MukBEF folds the chromosome of Escherichia coli and related bacteria. The SMC protein MukB dimerizes at its ‘‘hinge’’ domain, which connects via the long coiled-coil ‘‘arm’’ to the ABC-type ATPase ‘‘head’’ domain. The heads are bridged by the kleisin MukF, whereby the C-terminal winged-helix domain (cWHD) of MukF binds the ‘‘cap’’ surface of one MukB, and the N-terminal middle domain (MD) binds the coiled-coil ‘‘neck’’ of the other MukB. MukF also recruits the dimeric KITE protein MukE.

MukBEF is an obligate dimer, formed by two MukB2E2F monomers held together by their MDs and MukF N-terminal winged-helix domains (nWHDs). Focused sub-classification of the particle images revealed a DNA-bound structure. The DNA was captured directly at the open gate, while the proteins adopted a conformation virtually identical to the open-gate state. DNA-binding surfaces were largely contributed by MukE and MukF, and to a lesser extent by the root of the ν-MukB neck. The DNA was not entrapped inside the complex but bound at its periphery without contacting the top surface of the heads. As the captured DNA is positioned at the open neck gate but not entrapped, we reason that entrapment may be achieved by ingestion through the gate. We propose that the DNA-bound structure obtained here represents this capture state. Starting with the ATP- and DNA-bound capture state, we envision that upon ATP hydrolysis, the MukB subunits revert to their apo conformation. MukB is now free to sample the space around the DNA, and as its straightened neck is competent to bind the MD of MukF, the neck gate will eventually close. This results in an overall rotation of MukB that wraps MukF around the DNA and generates the holding state with DNA entrapped inside. Transition from the capture state to the holding state retains a short DNA segment at the center of the MukBEF dimer.

>[4x]MIERGKFRSLTLVNWNGFFARTFDLDELVTTLSGGNGAGKSTTMAAFVTALIPDLTLLHFRNTTEAGATSGSRDKGLHGKLRAGVCYSTLDVINSRHQRVVVGVRLQQVAGRDRKVDIKPFMIQGLPTAIQPTQLLTENVGERQARVLPLNELKDRLDEMEGVQFKQFNSITDYHAQMFDLGVIPKRLRSASDRSKFYRLIEASLYGGISSAITRSLRDYLLPENSGVRKAFQDMEAALRENRITLEAIRVTQSDRDLFKHLITEATSYVSADYMRHANERRTHLDEALALRGELFGSHKQLATEQYRHVEMARELAEQSGASSDLETDHQAASDHLNLVQTAMRQQEKIDRYQVDLEELSYRLEEQTDVVEEAGELQAEYEARTEATEQEVDELKSQLADYQQALDVQQTRAIQYQQALQALERARELCRLPDLSVDNAEEWLETFQAKEQQATEALLALEQKLSVADAAHNQFEQAYQLVKNIVGETSRSEAWQSARELLRDWPSQRHLADRVQPLRMRLSELEQRLNNQQNAERLLSEFCKRQGRQYQAEDLEALQNELEARQEALSLSVNEGGERRMEMRQELEQLKQKIQSLTARAPVWLAAQDTLNQLCEQSGETLASSNDVTEYMQQLLEREREATVERDEVAAQKRELEKQIERLSQPSGAEDSRMIALAERFGGVLLSEIYDDITIDDAPYFSALYGPARHGIVVPDLSLVRPHLETLEDCPEDLYLIEGDPQSFDDSVFNAEEQTNAVLVKSSDRQWRYSRYPELPLFGRAARENRLEALNLERDALAERYATLSFDVQKIQRAHQAFSQFVGKHLSVAFDTDPEAEIRELRQRHTELEREVSRFEDQTQQQRQQYAQAKESLTTLNRLIPQVTLLLDETLIDRVEEVREEMDEAQEAARFLQQHGSALTKLEPMVAVLQSDPQQHEQLQQDYETAKHSQHQAKQQAFALVEIVQRRVHFSYSDSAGMLSENADLNDKLRQRLEHAESDRSRAREQLRQQQAQYSQFNQVLASLKSSYETKQDMLKELLQEMKDIGVQADANAEMRARERRDRLHEALSVNRSRVNQLEKQIAFCEAEMENVQKKLRKLERDYYQIREQVVSAKAGWCAVMRMVKDNGVERRLHRRELAYMEGGALRSMSDKALGALRLAVADNEHLRDALRLSEDPKRPERKVQFFIAVYQHLRERIRQDIIRTDDPVDAIEQMEIELARLTEELTAREQKLAISSKSVANIIRKTIQREQNRIRMLNQGLQAVSFGQVRGVRLNVNVRESHAILLDVLSEQQEQHQDLFNSQRLTFSEAMAKLYQRLNPQVDMGQRLPQTIGEELLDYRNYLELDVEVNRGSDGWLKAESGALSTGEAIGTGMSILVMVVQSWEEESRRLRGKDISPCRLLFLDEAARLDAKSIATLFELCERLQMQLIIAAPENISPEKGTTYKLVRKVFKNHEHVHVVGLRGFGQDAPATQLISDVTA;>MSEYSQTVPELVSWARKNDFSISLPVERLAFLMAIAVLNSERLDGEMSEGELIDAFREVCKGFEQTAESVAVRANNAINDMVRQKLLNRFTSELADGNAIYRLTPLGISISDYYIRQREFSTLRLSMQLSIVANELHRAAEAAEEGGDEFHWHRNVFAPLKYSVAEIFDSIDMSQRLMDEQQNFVKEDIAALLNQDWQAAIANCEQLLSETSGTLRELQDTLEAAGDKLQANLLRIQDANMGSGGSELVDKLVFDLQSKLDRIISWGQQAIDLWIGYDRHVHKFIRTAIDMDKNRIFSQRLRQSVQHYFDNPWTLTVANAERLLDMRDEELALRNEEVTGELPLELEYEEFSEINDQLAAMIEKALLVYQQEQRPLDLGAVLRDYLAQHPLPRHFDVARILVDQAVRLGVAEADFSGLPAEWLAINDYGAKVQAHVIDTY[2x];>[4x]MSSTHIEQFMPVKLAQALANSLFPELDSQLRAGRHIGIDDLDNHAFLMDFQEQLEEFYARYNVELIRAPEGFFYLRPRSTTLIPRSVLSELDMMVGKILCYLYLSPERLANQGIFTSQELYEELISLADEGKLMKFVNQRSSGSDLDKQKLQEKVRTTLNRLRRLGMVYFLPNNNNKFTITEAVFRFGADVRSGDDPREIQLRMIRDGEAMPVEGSLSLDDSENDETPDNSAEGAGDEQP;>MSTIEERVKKIIGEQLGVKQEEVTNNASFVEDLGADXLDTVELVMALEEEFDTEIPDEEAEKITTVQAAIDYINGHQA[4x]5(R)-fluoro-beta-D-xylopyranose 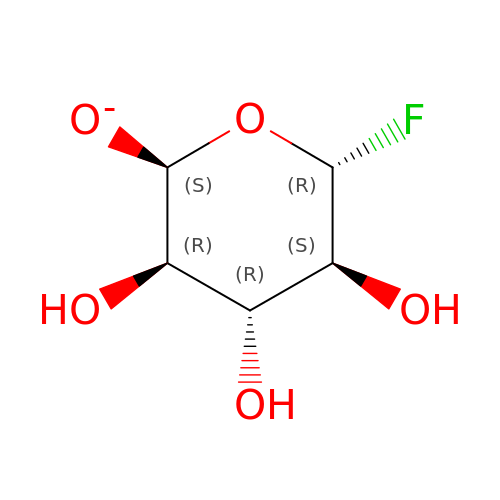| C5 H8 F O5 | CSWSGZBYLQUXQI-ZAMRNKCBSA-N>[4x]MGSSHHHHHHSSGMADLSELLKEGTKEAHDRAENTQFVKDFLKGNIKKELFKLATTALYFTYSALEEEMERNKDHPAFAPLYFPMELHRKEALTKDMEYFFGENWEEQVQC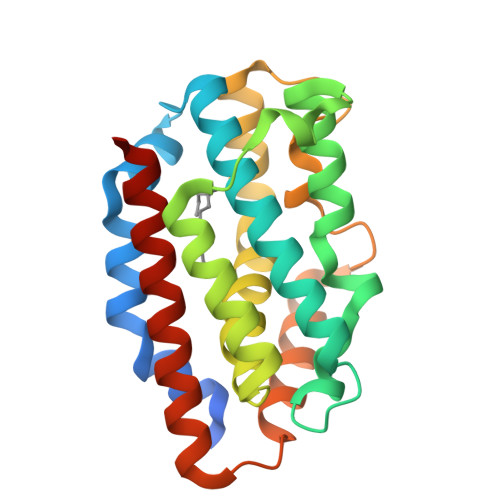PKAAQKYVERIHYIGQNEPELLVAHAYTRYMGDLSGGQVLKKVAQRALKLPSTGEGTQFYLFENVDNAQQFKQLYRARMNALDLNMKTKERIVEEANKAFEYNMQIFNELDQAGS> GPKTLHELLERIGLEEHTSTLLLNGYQTLEDFKELRETHLNELNIMDPQHRAKLLTAAELLLDY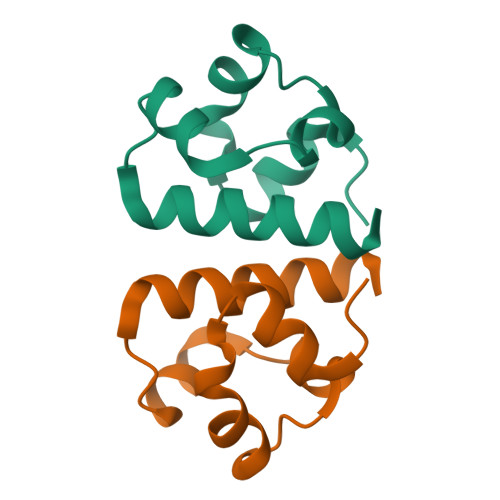D>QLSATILTDHQYLERTPLCAILKQKAPQQYRIRAKLRSYKPRRLFQSVKLHCPKCHLLQEVPHEGDLDIIFQDGATKTPDVKLQNTSLYDSKIWTTKNQKGRKVAVHFVKNNGILPLSNECLLLIEGGTLSEICKLSNKFNSVIPVRSGHEDLELLDLSAPFLIQGTIHHYGCKQCSSLRSIQNLNSLVDKTSWIPSSVAEALGIVPLQYVFVMTFTLDDGTGVLEAYLMDSDKFFQIPASEVLMDDDLQKSVDMIMDMFCPPG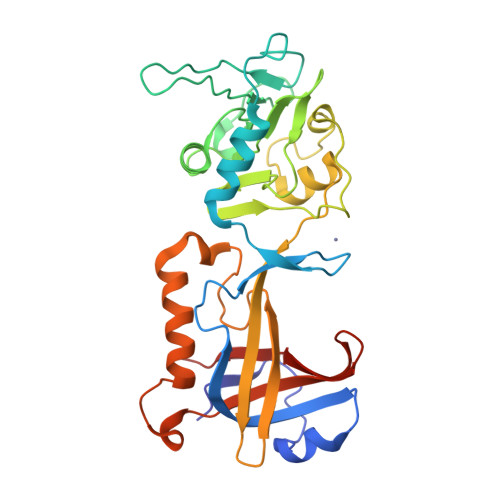IKIDAYPWLECFIKSYNVTNGTDNQICYQIFDTTVAEDVI[2x]> GGGRMSPEIALNRISPMLSPFISSVVRNGKVGLDATNCLRITDLKSGCTSLTPGPNCDRFKLHIPYAGETLKWDIIFNAQYPELPPDFIFGEDAEFLPDPSALHNLASWNPSNPECLLLVVKELVQQYHQFQCGRLRESSRLMFEYQTLLEEPQYGENMEIYAGKKNNWTGEFSARFLLKLPVDFSNIPTYLLKDVNEDPGEDVALLSVSFEDTEATQVYPKLYLSPRIEHALGGSSALHIPAFPGGGCLIDYVPQVCHLLTNKV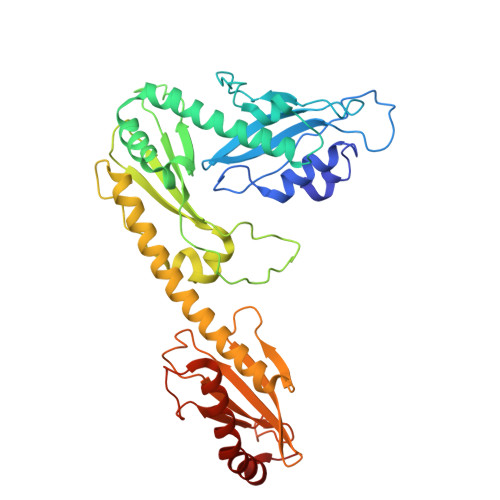QYVIQGYHKRREYIAAFLSHFGTGVVEYDAEGFTKLTLLLMWKDFCFLVHIDLPLFFPRDQPTLTFQSVYHFTNSGQLYSQAQKNYPYSPRWDGNEMAKRAKAYFKTFVPQFQEAAFANGKL> LGRTTRDDLINGNSASCADVIFIYARGSTETGNLGTLGPSIASNLESAFGKDGVWIQGVGGAYRATLGDNALPRGTSSAAIREMLGLFQQANTKCPDATLIAGGYSQGAALAAASIEDLDSAIRDKIAGTVLFGYTKNLQNRGRIPNYPADR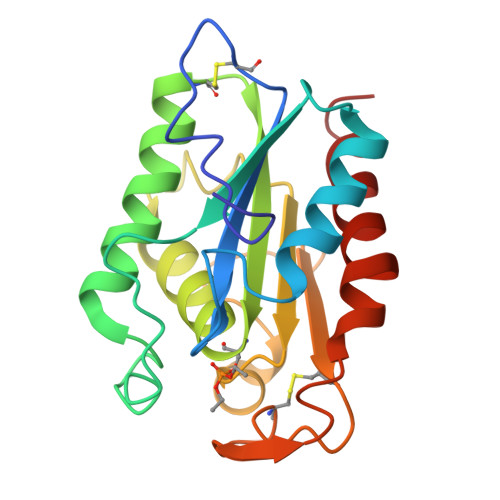TKVFCNTGDLVCTGSLIVAAPHLAYGPDARGPAPEFLIEKVRAVRG6-benzyl-3-hydroxythieno[2,3-d]pyrimidine-2,4(1H,3H)-dione | C13 H10 N2 O3 S 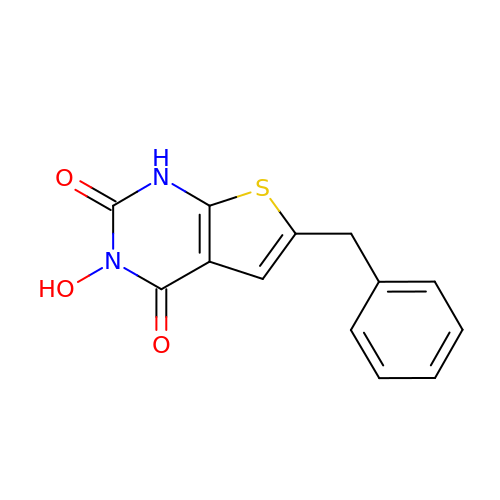| BATRIMGMBZXTOT-UHFFFAOYSA-N>[2x]GPLGSMSEEQVAQDTEEVFRSYVFYRHQQEQEAEGVAAPADPEMVTLPLQPSSTMGQVGRQLAIIGDDINRRYDSEFQ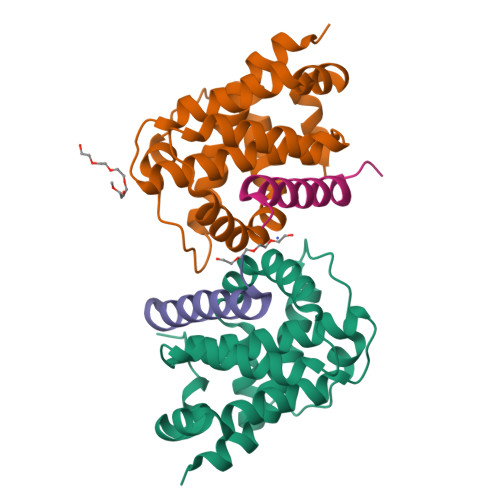TMLQHLQPTAENAYEYFTKIATSLFESGINWGRVVALLGFGYRLALHVYQHGLTGFLGQVTRFVVDFMLHHSIARWIAQRGGWVAALNLGNG;>[2x]DMRPEIWIAQELRRXGDEFNAYYARR> AIT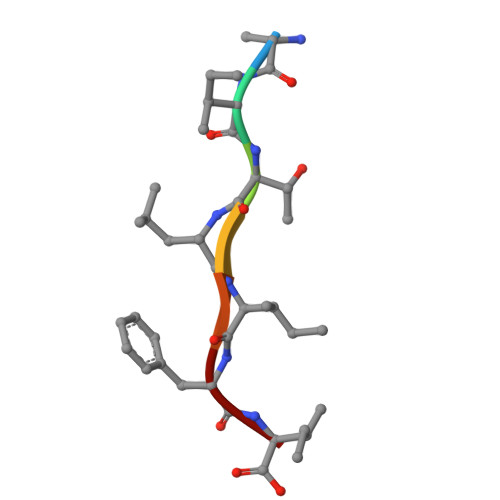LIFI> RKRHPDCDKPPDTKICQTVVR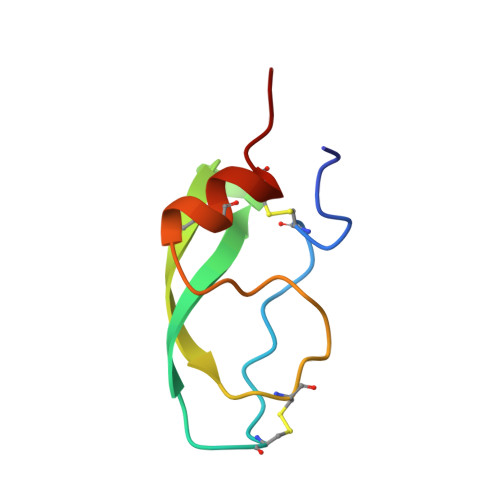AFYYKPSAKRCVQFRYGGCNGNGNHFKSDHLCRCECLEYR>MVLYFIGLGLYDERDITVKGLEIAKKCDYVFAEFYTSLMAGTTLGRIQKLIGKEIRVLSREDVELNFENIVLPLAKENDVAFLTPGDPLVATTHAELRIRAKRAGVESYVIHAPSIYSAVGITGLHI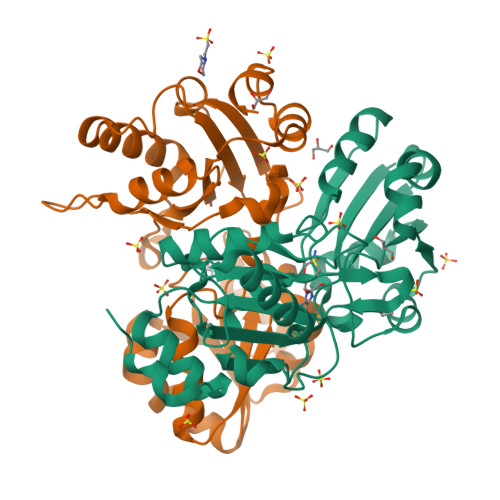YKFGKSATVAYPNGNWFPTSYYDVIKENAERGLHTLLFLDIKAEKRMYMTANEAMELLLKVEDMKKGGVFTDDTLVVVLARAGSLNPTIRAGYVKDLIREDFGDPPHILIVPGKLHIVEAEYLVEIAGAPREILRVNV[2x]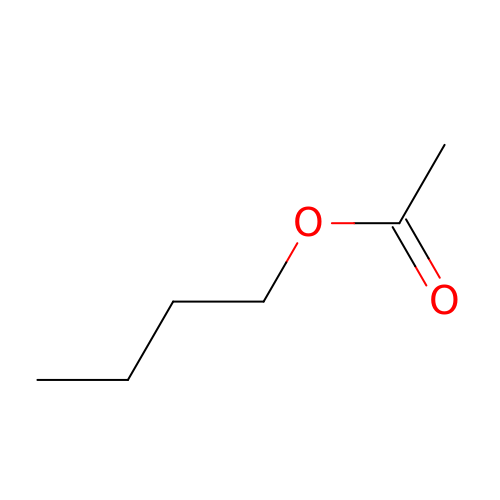butyl acetate | C6 H12 O2 | DKPFZGUDAPQIHT-UHFFFAOYSA-N>[2x]MATYLIGDVHGCYDELIALLHKVEFTPGKDTLWLTGDLVARGPGSLDVLRYVKSLGDSVRLVLGNHDLHLLAVFAGISRNKPKDRLTPLLEAPDADELLNWLRRQPLLQIDEEKKLVMAHAGITPQWDLQTAKECARDVEAVLSSDSYPFF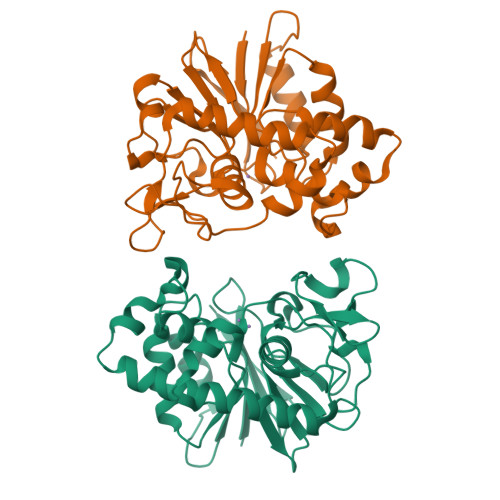LDAMYGDMPNNWSPELRGLGRLRFITNAFTRMRFCFPNGQLDMYSKESPEEAPAPLKPWFAIPGPVAEEYSIAFGHWASLEGKGTPEGIYALDTGCCWGGSLTCLRWEDKQYFVQPSNRHKDLGEAAAS> ENDVPAILKEIDSLVSREAVSAKEVSDAAVALTYLQVKANRRLWGKVLEKAGAAQDYDAASLTNLLWAINTGGVEHFKTVAELAGPAVSLLPSLSPVQLSIVVEALGGAGVKNYELYNKASAVVVSKIGEFKPAEIARVLYGVAFGGVNDVALAKAAGKVFASTEVDSRTAAQALYALAKLGRADKATVDALLKSFKKGTESASDAAAASFALGSLSFKAEKAIVDALKASAGDLAPAQAVEAAYGLALSGATDAEAFKALFGVVAPAIEKAPDALEVSSLAQLHVASTISGAKLPAAVGSFVAKAFGLAADAARLKRSSAESALVADVAAATAVAFGAQYRPEVASAVASYVKTAPDGSVLDIAITKGDAKVLVQAVPSSLLTSTTPAKPLGHVAAYSKVREAQGYAVAVVPANEFEALPDQKAKAQYVLAAIKKVAPSF;> ATEPAVSKKEVLYFLSSKDAESSTAVKSYLKSLYAGAQVEATETDASELIAQLEKKYLSAQVVEPGVHNIALPLGESGSAPVKRYAAELFNLGAQAGFECPFIEVSKKFGQETATSETVKDVLNKTKSYVSADYNAALNEVLSSVEAEINGPVLFDGKTEGFKKFAAKAKAVAVSRGLPADTILAYCAGSANEDAADKVSKEFFTWFESAYTADAAAEVKAIEAEAASILDRHLAKPVAQIRKEQASAYASLLKRAETAKGAKWAEKYLEDVKAVQWFDASVAEAPASGPKVAA;> MSSVRAGVEAGRRDLTTFTFSGLQDAPVAALSGSIKLNVAAKAGKAEVTVAAGAAKAATQVSAAALRKLSGSKISLAEVARISVLHSSIQNYLLSLSNERYQLLSQWPDFTTMYGKDFYYRAHPEDLKKFYDAADEYYKLYETVTEFDSLSALASQVVPNYAARRRSTVHPAIGSTVADGAFTNFLLSKQ;> MLARVASVALRRAEGKIMPQMVRALSVSAASAAQAELKLPTAPLQLSGTSAQIATLLWQVAAKENQLDKVQDELYQFIELFKQHSELRRLATDPFVPTLVRTKIISSVLKDSGASEITKKLFEALADEGALSALLEVTVNYEELMLAHKKEVYCTVITAEPLDKLERVELTKKAEKFVDAGFKLVMQEKIDKKLLGGFVIEFSDRRVDMSTAKKVEEFNNFVNKLVLSI;> MRSPAAFVARSGLFKASLGQSNWAQKAEQMMASVTRTFAADAKALDELRKPKFSSKYLIQHVSQKLIPAVKEWEKSYQPPVIHLGRVLSVGDGIARVYGLKSVQAGELVCFDSGVKGMALNLQADHVGVVVFGNDSVIHQGDLVYRTGQIVNVPIGPGTLGRVTDGLGQPIDGKGPLTNVRSSLVEVKAPGIIARQSVREPLFTGVKAVDALVPIGRGQRELIIGDRQTGKTAVAIDAIIHQKNCNEQVPKAQRVYCVYVAVGQKRSTVAQLVKLFTQTGAMRYTIMVSATASDAAPLQFLAPYSGCAMAEYFRDTGKHGLIIYDDLSKQSVAYRQMSLLLRRPPGREAFPGDVFYLHSRLLERAAKLSKELGGGSLTAFPVIETQAGDVSAYIATN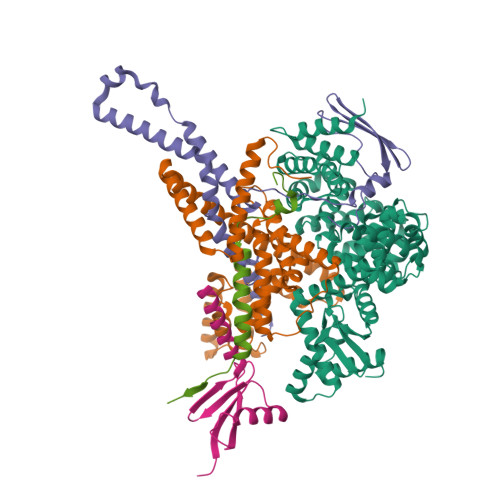VISITDGQIFLETELFYKGIRPALNVGLSVSRVGSAAQFPGMKQVAGTLKLELAQYREVAAFAQFGSDLDAATQYVLERGARLTEMLKQKQFAPIPIERQTVAVYAATKGFLDKVRVQDIVAAEEAVISQVNPAVFKILKANGKITPALDAHLKAELRKVKLPGA> AAAAAAMIVQRVVLNSRPGKNGNPVAENFRMEEVYLPDNINEGQVQVRTLYLSVDPYMRCRMNEDTGTDYITPWQLSQVVDGGGIGIIEESKHTNLTKGDFVTSFYWPWQTKVILDGNSLEKVDPQLVDGHLSYFLGAIGMPGLTSLIGIQEKGHITAGSNKTMVVSGAAGACGSVAGQIGHFLGCSRVVGICGTHEKCILLTSELGFDAAINYKKDNVAEQLRESCPAGVDVYFDNVGG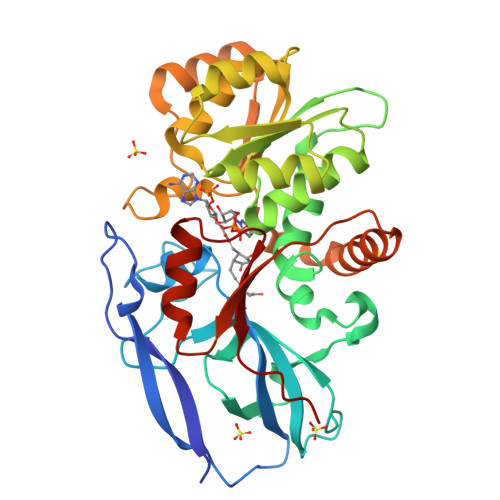NISDTVISQMNENSHIILCGQISQYNKDVPYPPPLSPAIEAIQKERNITRERFLVLNYKDKFEPGILQLSQWFKEGKLKIKETVINGLENMGAAFQSMMTGGNIGKQIVCISEEISL(R)-(3-aminopropyl)methylphosphinic 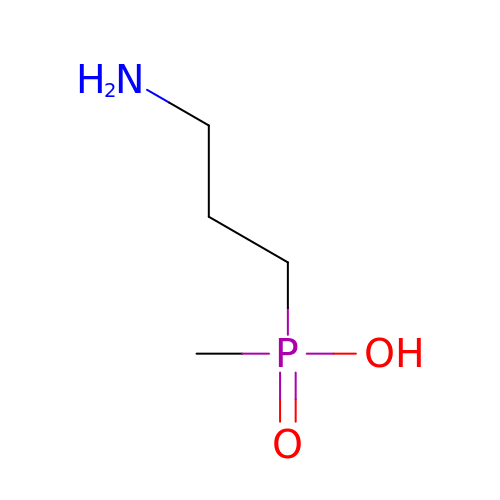acid | C4 H12 N O2 P | NHVRIDDXGZPJTJ-UHFFFAOYSA-N> PEGLSSEQQRAFLAVTQTPH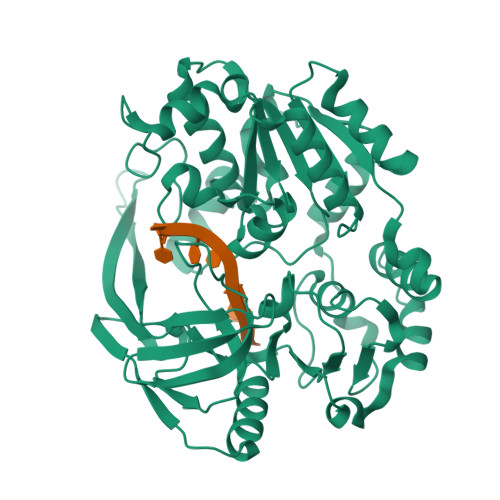PAHLITGPAGTGKTTLLYALQEFYKGRAVTLAPTGTAALQARGQTVHSFFRFPARLLRYRHPEDIRPPGPHSPLRKAIEQMEVLILDEVGMVRVDLLEAMDWALRKTRKRLEEPFGGVKVLLLGDTRQLEPVVPGGEEALYIARTWGGPFFFQAHVWEEVALRVHRLWESQRQREDPLFAELLKRLRQGDPQALETLNRAAVRPDGGEEPGTLILTPRRKEADALNLKRLEALPGKPLEYQAQVKGEFAETDFPTEAALTLKKGAQVILLRNDPLGEYFNGDLGWVEDLEAEALAVRLKRNGRRVVIRPFVWEKIVYTYDSEREEIKPQVVGTFRQVPVRLAWALTVHKAQGLTLDKVHLELGRGLFAHGQLYVALTRVRRLQDLSLSRPIAPTELLWRPEVEVFETRIQEGIWQKSHGWPSL>[4x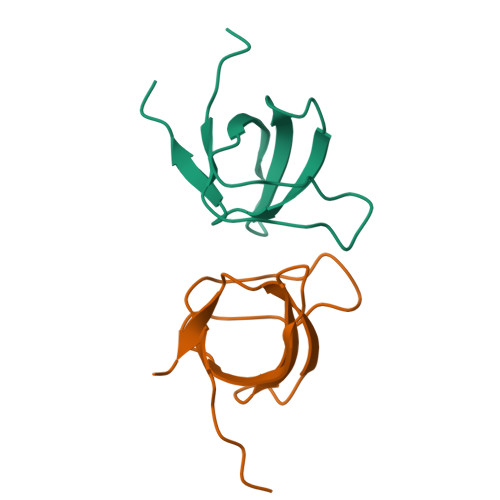]GHMEQTHRAIFRFVPRHEDELELEVDDPLLVELQAEDYWYEAYNMRTGARGVFPAYYAIEVTK> GPAFEFAVAMMKRNSSTVKTEYGEF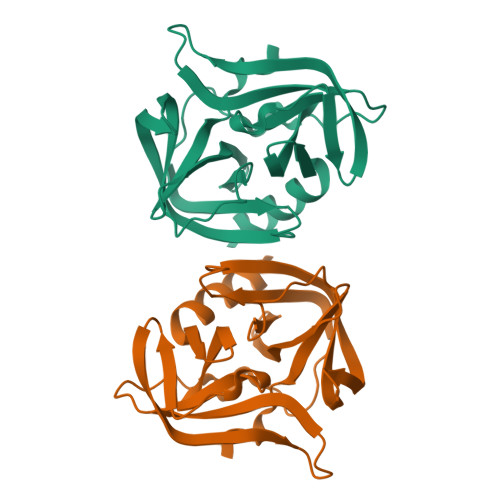TMLGIYDRWAVLPRHAKPGPTILMNDQEVGVLDAKELVDKDGTNLELTLLKLNRNEKFRDIRGFLAKEEVEVNEAVLAINTSKFPNMYIPVGQVTEYGFLNLGGTPTKRMLMYNFPTRAGQAGGVLMSTGKVLGIHVGGNGHQGFSAALLKHYFN>[2x]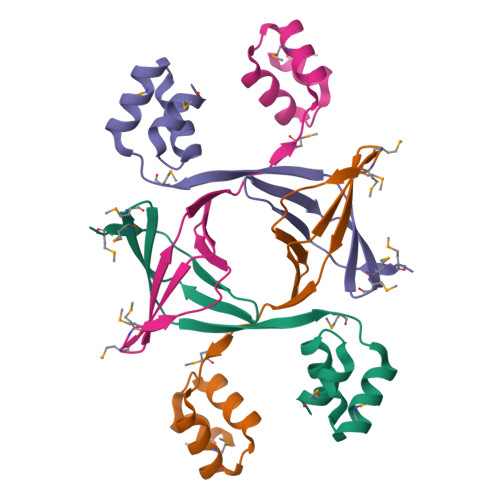GSHMKQMGMDMKDLRGVEEVVIKLKRKEIIIKNPKVNVMEFMGQKTYQVTGKARERSLEAEMEIPEDDIELVMNQTGASREDATRALQETGGDLAEAIMRLS> MPGPELSGW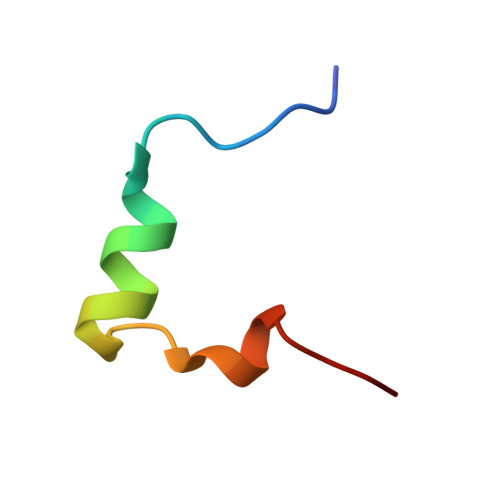ISEQLMTGRIPVSDIFCDI>LPTSNPAQELEARQLGRTTRDDLINGNSASCADVIFIYARGSTETGNLGTLGPSIASNLESAFGKDGVWIQGVGGAYRATLGDNALPRGTSSAAIREMLGLFQQANTKCPDATLIAGGYSQGAALAAASIEDLDSAIRDKIAGTVLFGYTKNLQNRGRIPNYPADRTKVFCKTGDLVCTGSL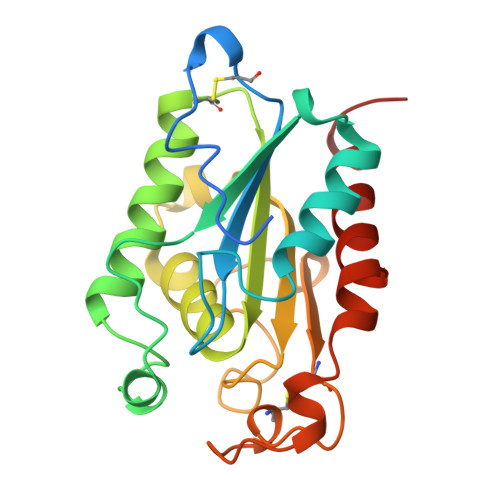IVAAPHLAYGPDAEGPAPEFLIEKVRAVRGSA[3x]> MKDVTIIGGGPSGLYASFYAGLRDMSVRLIDVQSELGGKMRIYPEKIIWDIGGIAPKPCHEILKDTIKQGLYFKPEVHLNERVVDIRKKAERHFEVETEAGEIYTSKAVIIAIGAGIINPKQLDVKGVERYQLTNLHYVVQSYRRFKDKDVLISGGGNTALDWAHDIAKIAKSVTVVYRKEDVSGHEAMKTLVTDLNVKLCPKTRIKYLVGNDDETH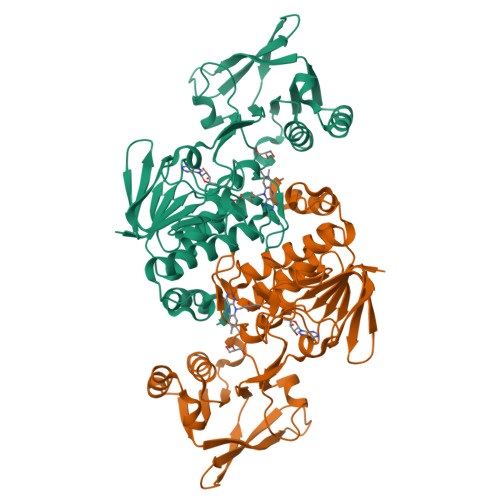ISEVVLEHVESGDRHTVKFDDVIISHGFDRCNTLLSETSSKLDMHDDCRVKGFGNTTTSIPGIYACGDIVYHDAKSHLIASAFSDGANAANLAKTYIQPDANAEGYVSSHHEVFKEANKTIVNKHLY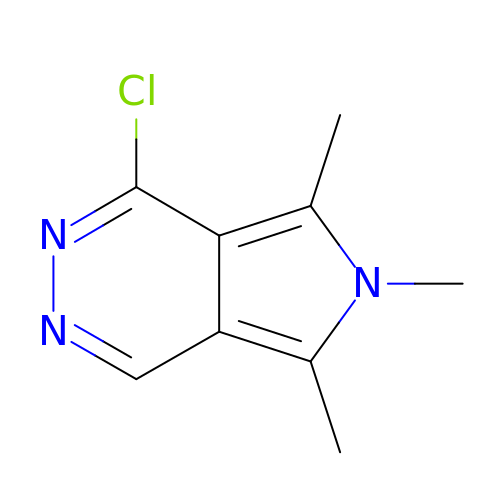4-chloranyl-5,6,7-trimethyl-pyrrolo[3,4-d]pyridazine | C9 H10 Cl N3 | RIVWEUYBKRJSIF-UHFFFAOYSA-N>[2x]MAFHEVRFPANLSFGSVGGPERRTEIVTLSSGHEERNSPWAHSRRHYDAGVGL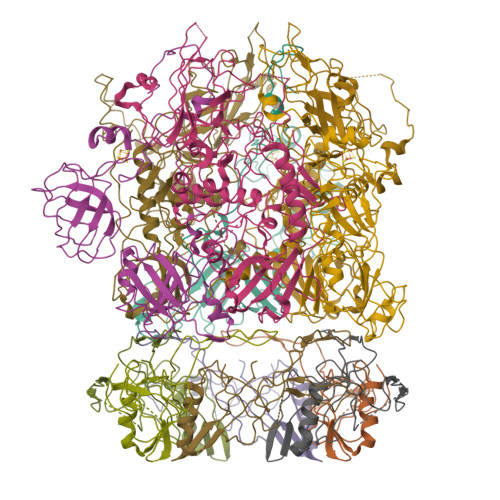RSLDDVERLIAFFEARGGQLHGFRWKDWADFKSCPASRAVAHEDQLIGMGDGVTTAFQLVKTYVSGGQSYLRPIVKPVEGTVKLGIAGDHQAEAVNFAVDHATGIVSFNEPPPQGARVTAGFEFDVPVRFDTDRIAVSVQSFQAGDLPQVPVVEVRI;> MAYPESLKAHLQGGVTTLARAWALARADGRVLGFTDHDVVLRFDGISFEPGSGMTAKAVLQGTGLSVDNTESYGALSSEAITEADLLAGRYDGAAVTVWLVNWADPAMRAVIFRGHLGEVSRGAGAFTAELRGLTAALGQEQGRIYHPRCAAVLGDGRCRFDLTKDGYALEAALGGVDEAVVLRLAEGAGFEDRWFEKGRLVVLDGAAAGLIGVVKNDRLQADGSRLIELWQRLGANPVAGDRVRIEPGCDKRAGTCRLKFDNFLNFRGFPHIPGEDWMVSYPVQSGTNDGGSLFR;> MATILLSAAGAAIGGGFGGTVLGLSGAVIGRAVGATLGRVIDQRLLGSGSQSVETGRVDRLRLSSASEGEAVGRLWGRMRVAGQVIWATRFFESASVEKSGKGVPRATVTSYSYSLSLALALCEGEILRVGRVWADGSEIEVSGLNMRVYRGGEDQLPDPKIAAVEGAEAAPAYRGIAYVVLEDLQLAPFGNRVPQFTFEVVRAAQGALAEAEPDLTRGLRAVALIPGTGEYALATTPVYLATGSGVTATQGVANQNAPGGQTDLVAALERLDEELPNCGAVSLVVSWFGDDLRCGACDVKPKVASVAEEGANMPWRVAGLERAGAEEVPRLSGQSVYGGTPADAAVIEAIAALRAAGKAVTFYPFILMAQLAGNGLPDPWNPGSAQPALPWRGRITLSVAPGRAGSPDGTAAAEAQVAGFFGAASPGDSAIAGGEVVYSGPEEWSMRRFILHYAHLCQLAGGVDAFCIGTEMVALTQIRGPSNSFPAVAAFRQLAGEVKAILGPGCKIGYAADWSEYWGYAPGNGERFFHLDPLWADENIDFIGIDNYLPLSDWRDGADHADAGWGSIHALDYLRSNIEGGEYYDWFYAAPEHRAAQIRTPITDGDHDEPWIWRAKDLRNWWLNDHHERVGGLRSEVATAWVPQSKPIWFTEMGCAAIDKGTNQPNKFLDPKSSESGLPHHSDGRRDELIQMQYLRAMTGYWGEAARNPVSAVYGGPMLDMSRAHVWAWDARPWPQFPLNTALWSDGENYARGHWISGRAVAQPLASVVAEICGAAGITEIDVSGLYGLVRGYTMTGDQTGRAGLQALMLAYGFEALERDGQLVFRMRDGRVAADLAAADLALGEGEAVVETVRAAEAEIAGRVRLAYVEAEGDFEVKAVEAVFPDAAAGAAAGSELSLALTRAQAQGIVGRWLAEARVARDTARFALPPSRGHLGTGDVVRLDLPEGKRRYRIDRVEQAGLIQVEAVRVEPGIYAPADEVEDPASLRPFAAPVPVTAVFLDLPLMKGDEDPVAPHLAVTATPWPGTVAVWSSDEDAGYALNASLGTRAVIGQTLTPLFRARPGVWDRGAALRVRLASGALDSATAAKVLNGANAMAIGDGSSENWEVFQFAEAALVEGKIWDISLRLRGQLGTDALMPEVWPEGSVVVALNGAPEQILLPSAARGLARHYRIGAAVRSYDDPSFVHRIEAFAGAGLRPFSPCHLRAEPGASGWAFRWVRRTRIDGDSWQGYEVPLGETAELYLVRVLEGTAVKREVTVGEASWSYPAALQAADGIAGAFTLEVAQVSDVYGPGLAARITVGA> PKHGKRYRALLEKVDPNKIYTIDEAAHLVKELATAKFDETVE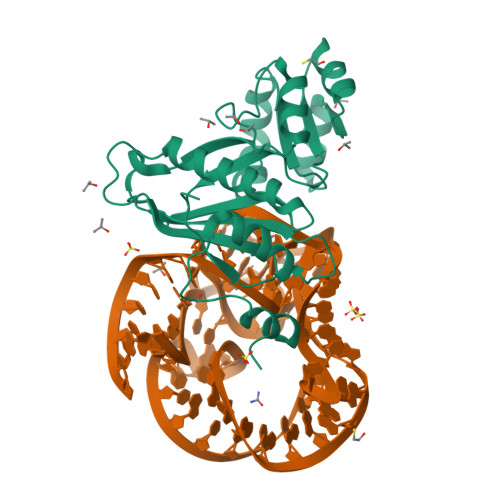VHAKLGIDPRRSDQNVRGTVSLPHGLGKQVRVLAIAKGEKIKEAEEAGADYVGGEEIIQKILDGWMDFDAVVATPDVMGAVGSKLGRILGPRGLLPNPKAGTVGFNIGEIIREIKAGRIEFRNDKTGAIHAPVGKASFPPEKLADNIRAFIRALEAHKPEGAKGTFLRSVYVTTTMVPSVRINPHS> VDWTDAERSAIVGLWGKISVDEIGPQALARLLIVSPWTQRHFSTFGNLSTPAAIMGNPAVAKHGKTVMHGLDRAVQNLDDIKNTYVTLSVMHSEKLFVDPDNFRLLADCITVCVAAKLGP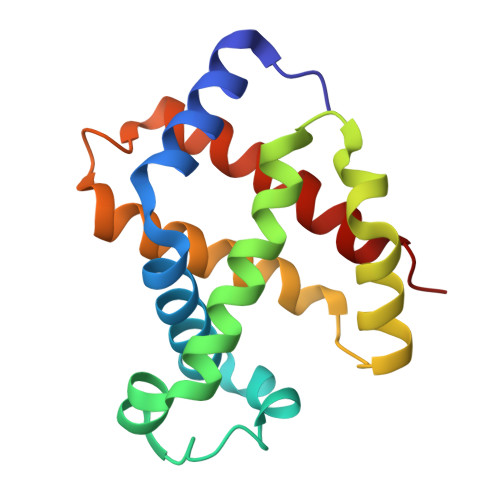AVFSADTQEAFQKFLAVVVSALGRQYH4-{8-amino-3-[(6R,8aS)-3-oxo-3,5,6,7,8,8a-hexahydroindolizin-6-yl]imidazo[1,5-a]pyrazin-1-yl}-3-methoxy-N-[4-(trifluoromethyl)pyridin-2-yl]benzamide | C28 H26 F3 N7 O3 | 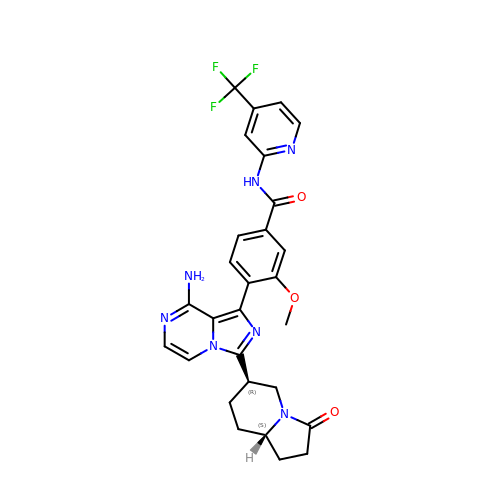OMIQRSKHABIPRH-AEFFLSMTSA-N> SIDSALNWDGEMTVTRFDSMTGAHFVIRLDSTQLGPAAGGTRAAQYSNLADALTDAGKLAGAMTLKMAVSNLPMGGGKSVIALPAPRHSIDPSTWARILRIHAENIDKLSGNYWTGPDVNTNSADMDTLNDTTEFVFGRSLERGGAGSSAFTTAVGVFEAMKATVAHRGLGSLDGLTVLVQGLGAVGGSLASLAAEAGAQLLVADTDTERVAHAVALGHTAVALEDVLSTPCDVFAPCAMGGVITTEVARTLDCSVVAGAANNVIADEAASDILHARGILYAPDFVANAGGAIHLVGREVLGWSESVVHERAVAIGDTLNQVFEISDNDGVTPDEAARTLAGRRAREASTTTATA;> SIDSALNWDGEMTVTRFDKMTGAHFVIRLDSTQLGPAAGGTRAAQYSQLADALTDAGKLAGAMTLKMAVSNLPMGGGKSVIALPAPRHSIDPSTWARILRIHAENIDKLSGNYWTGPDVNTNSADMDTLNDTTEFVFGRSLERGGAGSSAFTTAVGVFEAMKATVAHRGLGSLDGLTVLVQGLGAVGGSLASLAAEAGAQLLVADTDTERVAHAVALGHTAVALEDVLSTPCDVFAPCAMGGVITTE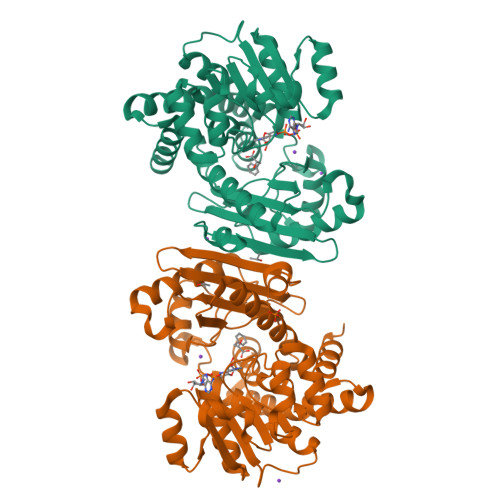VARTLDCSVVAGAANNVIADEAASDILHARGILYAPDFVANAGGAIHLVGREVLGWSESVVHERAVAIGDTLNQVFEISDNDGVTPDEAARTLAGRRAREASTTTATA>MIFTNAILVISALLPATVLSLQHTEDSLFPARCWPDPCAGITFQNDTYVCGDPRLGPVVLPQKFPLNNELRTYARFGALCPAEFLDKWATDVAPNGTYIYPPANGFALDTEEQPILGNATLPVGMKLDRFGSEYGTFLAPLGAPYIERSLPPSNLNTFDGMYPYNYHVYQVTKEFVVGLGPIAPWFEQPGMGTQFVTYTNVLGLIDDGYLRRLDESEYAAKVEYSNPYTPGPNQDVLFQGPGHHHHHH[4x]

The majority of cellular NAD+ is generated in the salvage pathway, where the Nam released in signaling reactions is resynthesized into NAD+.4 Given its importance, NAD+ is targeted by toxins from many pathogenic microorganisms, including Streptococcus pyogenes and Mycobacterium tuberculosis. These toxins invade cells and act as NAD glycohydrolases, cleaving NAD+ into Nam and ADPR and rapidly depleting the cellular NAD pool, ultimately leading to cell death. In this context, we recently discovered a new fungal NADase on the surface of conidia from Aspergillus fumigatus (AfNADase), the predominant etiologic agent of Aspergillosis. The catalytic part of the TNT is structurally highly similar to AfNADase. Intriguingly, the active site architecture of the bacterial and fungal enzymes is conserved, but their structural superimposition reveals the presence of a unique C-terminal calcium-binding motif in AfNADase, which is located at the edge of the dimerization interface. In the present study, we addressed the structural and functional role of calcium binding by introducing mutations in the C-terminus of AfNADase that precluded the binding of the metal ion.

In the first variant, we abolished calcium binding by mutating two critical residues for metal ion coordination into alanine (D219A/E220A), referred to here as AfNADaseD219A/E220A. Interestingly, the KM (88.3 ± 12.2 μM) and Vmax (2956 ± 157 μmol/min/mg) of AfNADaseD219A/E220A were far less affected than the AfNADase NcC-Term. The ASU contained two homodimers, which were lacking Ca2+ ions as expected. A closer inspection revealed that one dimer represented the native-like conformation, whereas the other had a conformation with an unfolded C-terminus. Superimposition of the dimers to AfNADase (C alpha) showed RMSD of 0.25 and 1.00 for chain AB (native-like) and chain CD (unfolded C-terminus), respectively. Dimer 1 has a C-terminus folded in a manner identical to that of AfNADase with the characteristic helix-turn-helix motif for the Ca2+-binding site, allowing the C-terminus to intertwine on the surface of the complementary protomer participating in dimer formation. In contrast, in dimer 2, the C-terminal region, including the mutated Ca2+-binding site, is unfolded, causing the C-terminus to turn ∼45° and lose the interactions with the complementary protomer of the dimer. The two α-helixes, forming part of the dimerization interface of AfNADase8 and dimer 1 of AfNADaseD219A/E220A, are unfolded in dimer 2 and rather form a loop-to-loop interaction. In dimer 2, the entire catalytic domain translocates ca. 2 Å away from the dimerization interface, also showing major rearrangements in the loop (156NTFDGMYPY164) containing residues Phe158 and Tyr164 8 that were earlier observed to be important for substrate binding.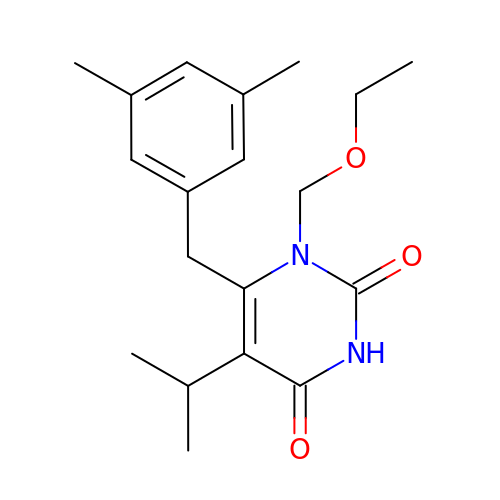6-(3',5'-DIMETHYLBENZYL)-1-ETHOXYMETHYL-5-ISOPROPYLURACIL | C19 H26 N2 O3 | NVGVZWUORYLPAL-UHFFFAOYSA-N>QEVEFDIPPQALGSALQEFGRQADIQVLYRPEEVRNKRSSAIKGKLEPNQAITELLRGTGASVDFQGNAITISVAEAADSSVDLGATMITSNQLGTITEDSGSYTPGTIATATRLVLTPRETPQSITVVTRQNMDDFGLNNIDDVMRHTPGITVSAYDTDRNNYYARGFSINNFQYDGIPSTARNVGYSAGNTLSDMAIYDRVEVLKGATGLLTGAGSLGATINLIRKKPTHEFKGHVELGAGSWDNYRSELDVSGPLTESGNVRGRAVAAYQDKHSFMDHYERKTSVYYGILEFDLNPDTMLTVGADYQDNDPKGSGWSGSFPLFDSQGNRNDVSRSFNNGAKWSSWEQYTRTVFANLEHNFANGWVGKVQLDHKINGYHAPLGAIMGDWPAPDNSAKIVAQKYTGETKSNSLDIYLTGPFQFLGREHELVVGTSASFSHWEGKSYWNLRNYDNTTDDFINWDGDIGKPDWGTPSQYIDDKTRQLGSYMTARFNVTDDLNLFLGGRVVDYRVTGLNPTIRESGRFIPYVGAVYDLNDTYSVYASYTDIFMPQDSWYRDSSNKLLEPDEGQNYEIGIKGEYLDGRLNTSLAYFEIHEENRAEEDALYNSKPTNPAITYAYKGIKAKTKGYEAEISGELAPGWQVQAGYTHKI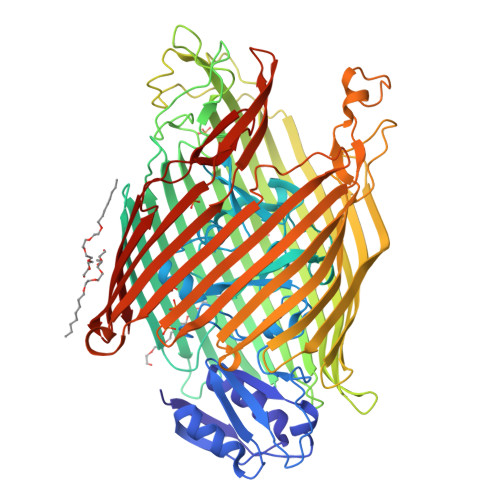IRDDSGKKVSTWEPQDQLSLYTSYKFKGALDKLTVGGGARWQGKSWQMVYNNPRSRWEKFSQEDYWLVDLMARYQITDKLSASVNVNNVFDKTYYTNIGFYTSASYGDPRNLMFSTRWDF[2x];> SKGKKKS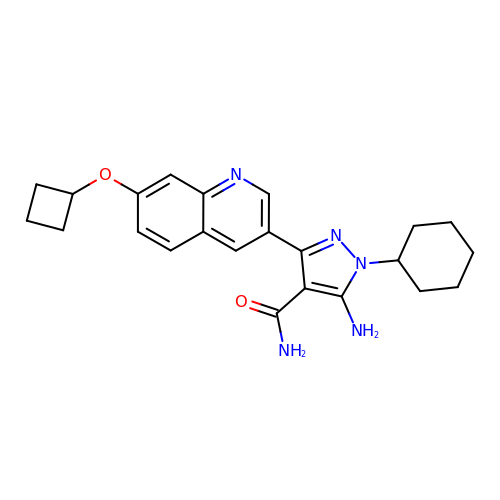5-amino-3-[7-(cyclobutyloxy)quinolin-3-yl]-1-cyclohexyl-1H-pyrazole-4-carboxamide | C23 H27 N5 O2 | AJQKERUGIYLYDN-UHFFFAOYSA-N>MASNEGVENRPFPYLTVDADLLSNLRQSAAEGLFHSFDLLVGKDAREAGIKFEVLLGVYTNAIQYVRFLETALAVSCVNTEFKDLSRMTDGKIQFRISVPTIAHGDGRRPSKQRTFIVVKNCHKHHISTEMELSMLDLEILHSIPETPVEYAEYVGAVKTVASALQFGVDALERGLINTVLSVKLRHAPPMFILQTLADPTFTERGFSKTVKSDLIAMFKRHLLEHSFFLDRAENMGSGFSQYVRSRLSEMVAAVSGESVLKGVSTYTTAKGGEPVGGVFIVTDNVLRQLLTFLGEEADNQIMGPSSYASFVVRGENLVTAVSYGRVMRTFEHFMARIVDSPEKAGSTKSDLPAVAAGVEDQPRVPISAAVIKLGNHAVAVESLQKMYNDTQSPYPLNRRMQYSYYFPVGLFMPNPKYTTSAAIKMLDNPTQQLPVEAWIVNKNNLLLAFNLQNALKVLCHPRLHTPAHTLNSLNAAPAPRDRRETYSLQHRRPNHMNVLVIVDEFYDNKYAAPVTDIALKCGLPTEDFLHPSNYDLLRLELHPLYDIYIGRDAGERARHRAVHRLMVGNLPTPLAPAAFQEARGQQFETATSLAHVVDQAVIETVQDTAYDTAYPAFFYVVEAMIHGFEEKFVMNVPLVSLCINTYWERSGRLAFVNSFSMIKFICRHLGNNAISKEAYSMYRKIYGELIALEQALMRLAGSDVVGDESVGQYVCALLDPNLLPPVAYTDIFTHLLTVSDRAPQIIIGNEVYADTLAAPQFIERVGNMDEMAAQFVALYGYRVNGDHDHDFRLHLGPYVDEGHADVLEKIFYYVFLPTCTNAHMCGLGVDFQHVAQTLAYNGPAFSHHFTRDEDILDNLENGTLRDLLEISDLRPTVGMIRDLSASFMTCPTFTRAVRVSVDNDVTQQLAPNPADKRTEQTVLVNGLVAFAFSERTRAVTQCLFHAIPFHMFYGDPRVAATMHQDVATFVMRNPQQRAVEAFNRPEQLFAEYREWHRSPMGKYAAECLPSLVSISGMTAMHIKMSPMAYIAQAKLKIHPGVAMTVVRTDEILSENILFSSRASTSMFIGTPNVSRREARVDAVTFEVHHEMASIDTGLSYSSTMTPARVAAITTDMGIHTQDFFSVFPAEAFGNQQVNDYIKAKVGAQRNGTLLRDPRTYLAGMTNVNGAPGLCHGQQATCEIIVTPVTADVAYFQKSNSPRGRAACVVSCENYNQEVAEGLIYDHSRPDAAYEYRSTVNPWASQLGSLGDIMYNSSYRQTAVPGLYSPCRAFFNKEELLRNNRGLYNMVNEYSQRLGGHPATSNTEVQFVVIAGTDVFLEQPCSFLQEAFPALSASSRALIDEFMSVKQTHAPIHYGHYIIEEVAPVRRILKFGNKVVF[4x];>[4x]MARRLPKPTLQGRLEADFPDSPLLPKFQELNQNNLPNDVFREAQRSYLVFLTSQFCYEEYVQRTFGVPRRQRAIDKRQRASVAGAGAHAHLGGSSATPVQQAQAAASAGTGALASSAPSTAVAQSATPSVSSSISSLRAATSGATAAASAAAAVDTGSGGGGQPHDTAPRGARKKQ;>MKVQGSVDRRRLQRRIAGLLPPPARRLNISRGSEFTRDVRGLVEEHAQASSLSAAAVWRAGLLAPGEVAVAGGGSGGGSFSWSGWRPPVFGDFLIHASSFNNAEATGTPLFQFKQSDPFSGVDAVFTPLSLFILMNHGRGVAARVEAGGGLTRMANLLYDSPATLADLVPDFGRLVADRRFHNFITPVGPLVENIKSTYLNKITTVVHGPVVSKAIPRSTVKVTVPQEAFVDLDAWLSGGAGGGGGVCFVGGLGLQPCPADARLYVALTYEEAGPRFTFFQSSRGHCQIMNILRIYYSPSIMHRYAVVQPLHIEELTFGAVACLGTFSATDGWRRSAFNYRGSSLPVVEIDSFYSNVSDWEVIL[2x];>[4x]MDLKVVVSLSSRLYTDEIAKMQQRIGCILPLASTHGTQNVQGLGLGQVYSLETVPDYVSMYNYLSDCTLAVLDEVSVDSLILTKIVPGQTYAIKNKYQPFFQWHGTGSLSVMPPVFGREHATVKLESNDVDIVFPMVLPTPIAEEVLQKILLFNVYSRVVMQAPGNADMLDVHMHLGSVSYLGHHYELALPEVPGPLGLALLDNLSLYFCIMVTLLPRASMRLVRGLIRHEHHDLLNLFQEMVPDEIARIDLDDLSVADDLSRMRVMMTYLQSLASLFNLGPRLATAAYSQETLTATCWLR;> MDVHIDNQVLSGLGTPLLVHLFVPDTVMAELCPNRVPNCEGAWCQTLFSDRTGLTRVCRVFAARGMLPGRPSHRGTFTSVPVYCDEGLPELYNPFHVAALRFYDEGGLVGELQIYYLSLFEGAKRALTDGHLIREASGVQESAAAMQPIPIDPGPPGGAGIEHMPVAAAQVEHPKTYDLKQILLEITQEENRGEQRLGHAGSPALCLGLRLRAGAETKAAAETSVSKHHPALENPSNIRGSAGGEGGGGRAGTGGTVGVGSGALSRVPVSFSKTRRAIRESRALVRGIAHIFSPHALYVVTYPELSAQGRLHRMTAVTHASPATDLAEVSILGAPEREFRFLISVALRISASFREKLAMQAWTAQQEIPVVIPTSYSRIYKNSDLIREAFFTVQTRVSWESCWVKATISNAPKTPDACLWIDSHPLYEEGASAWGKVIDSRPPGGLVGAASQLVALGTDGHCVHLATTSDGQAFLVLPGGFVIKGQLALTPEERGYILARHGIRREQ;>[2x]MALSGHVLIDPARLPRDTGPELMWAPSLRNSLRVSPEALELAEREAERARSERWDRCAQVLKNRLLRVELDGIMRDHLARAEEIRQDLDAVVAFSDGLESMQVRSPSTGGRSAPAPPSPSPAQPFTRLTGNAQYAVSISPTDPPLMVAGSLAQTLLGNLYGNINQWVPSFGPWYRTMSANAMQRRVFPKQLRGNLNFTNSVSLKLMTEVVAVLEGTTQDFFSDVRHLPDLQAALILSVAYLLLQGGSSHQQRPLPASREELLELGPESLEKIIADLKAKSPGGNFMILTSGNKEARQSIAPLNRQAAYPPGTFADNKIYNLFVGAGLLPTTAALNVPGAAGRDRDLVYRIANQIFGEDVPPFSSHQWNLRVGLAALEALMLVYTLCETANLAEAATRRLHLSSLLPQAMQRRKPAMASAGMPGAYPVQTLFRHGELFRFIWAHYVRPTVAADPQASISSLFPGLVLLALELKLMDGQAPSHYAINLTGQKFDTLFEIINQKLLFHDPAAMLAARTQLRLAFEDGVGVALGRPSPMLAAREILERQFSASDDYDRLYFLTLGYLASPVAPS;>MSNGDWGQSQRTRGTGPVRGIRTMDVNAPGGGSGGSALRILGTASCNQAHCKFGRFAGIQCVSNCVLYLVKSFLAGRPLTSRPELDEVLDEGARLDALMRQSGILKGHEMAQLTDVPSSVVLRGGGRVHIYRSAEIFGLVLFPAQIANSAVVQSLAEVLHGSYNGVAQFILYICDIYAGAIIIETDGSFYLFDPHCQKDAAPGTPAHVRVSTYAHDILQYVGAPGAQYTCVHLYFLPEAFETEDPRIFMLEHYGVYDFYEANGSGFDLVGPELVSSDGEAAGTPGADSSPPVMLPFERRIIPYNLRPLPSRSFTSDSFPAARYSPAKTNSPPSSPASAAPASAAPASAAPASAAPASAAPASAAPASAAPASAAPASSPPLFIPIPGLGHTPGVPAPSTPPRASSGAAPQTPKRKKGLGKDSPHKKPTSGRRLPLSSTTDTEDDQLPRTHVPPHRPPSAARLPPPVIPIPHQSPPASPTPHPAPVSTIAPSVTPSPRLPLQIPIPLPQAAPSNPKIPLTTPSPSPTAAAAPTTTTLSPPPTQQQPPQSAAPAPSPLLPQQQPTPSAAPAPSPLLPQQQPPPSAARAPSPLPPQQQPLPSATPAPPPAQQLPPSATTLEPEKNHPPAADRAGTEISPSPPFGQQPSFGDDASGGSGLVRYLSDLEEPFLSMSDSEEAESDLASDIPTTEDEDMFEDEVFSNSLESGSSAPTSPITLDTARSQYYQTTFDIETPEMDFVPLESNIARIAGHTYQEQAIVYDPASNREVPEADALSMIDYLLVTVVLEQGLIRSRDRSSVLNLLEFLKDWSGHLQVPTLDLEQLLTSELNIQNLANMLSENKGRAGEFHKHLAAKLEACLPSLATKDAVRVDAGAKMLAEIPQLAESDDGKFDLEAARRRLTDLLSGGDQEAGEGGGEPEDNSIYRGPHVDVPLVLDDESWKRLLSLAEAARTAVARQQAGVDEEDVRFLALLTAIEYGAPPAASVPPFVHNVAVRSKNAALHVRRCTADIRDKVASAASDYLSYLEDPSLPTVMDFDDLLTHLRHTCQIIASLPLLNIRYTSIEWDYRELLYLGTALSDMSGIPWPLERVEEDDPSIAPLPEFETVAKKQKELETTRENEKRLRTILDDIEAMLGLAGVASAPGAPISPASPSATPANHDNPEATPPLADTAALTIPVIEKYIANAGSIVGAAKNPTYIRLRDTIQQIVRSKKYLMNILKSITFYTIDNYIASFEESIDHLYRDLPVLDPEVQDGIDRILDPMVSEALHTFEMGNRLTLEPARLVALQNFATHSTLKETAAAVNLLPGLLAVYDATITGQAPEDALRLLSGLQNQLSQTLIPGKLKKRFLSYLQKLKNNNNDQLRQKEVQAWRLEAEGFKPATEEQLEAFLDTAPNKELKRQYEKKLRQLMETGRKEKEKLREQEDKERQERRAREANEAWARIRKALGARPEPAPTSPDDWNTLLASLLPDNTDSAAAAAAAVARNTDILDSLTQILAAMLLGITRVRRERLRSLLVDDGGAAERMEAAEPGWFTDIETGPLARLDAWPATPAATAKEGGGGRGAEEAAGALFRARTAADAIRSALAQTRQALQSPDMKSAVVNTDLEAPYAEYERGLAGLLEKRRAAEAALTAIVSEYVDRTLPEATNDPGQANLPPPPTIPQATAPPRLASDSALWPKKPQLLTRRERDDLLQATGDFFSELLTEAEAAEVRALEEQVRESQTLMAKAHEMAASTRRGFHTALEAVLSRSRDEAPDDELRSLLPSPPKAPVQAPLEAALARAAAGNGSWPYRKSLAAAKWIRGICEAVRGLSEGALALAGGAGAWLNLAAAADGEIHELTRLLEVEGMAQNSMDGMEELRLALATLDPKRVAGGKETVADWKRRLSRLEAIIQEAQEESQLQGTLQDLVTQARGHTDPRQLKIVVEAAR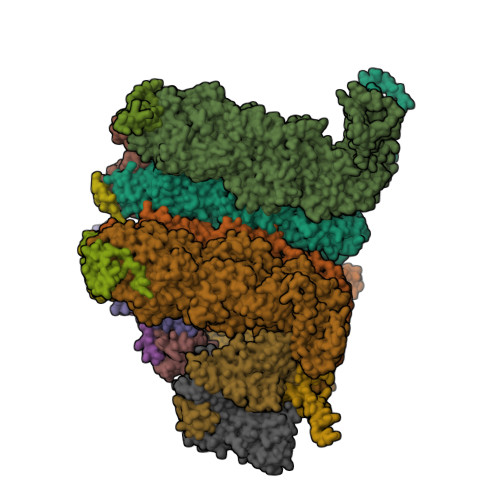GLALGASAGSQYALLKDKLLRYASAKQSFLAFYETAQPTVFVKHPLTNNLPLLITISAPPTGWGNGAPTRRAQFLAAAGPAKYAGTLWLETESPCDPLNPAYVSADTQEPLNYIPVYHNFLEYVMPTVLENPEAFSLTPAGRPQAIGPPQDDQERRRRTLASVASARLSAAAADSYWDTWPDVESNAGELLREYVSAPKALMEDLADNPIVAMTLLAHASLIASRNHPPYPAPATDREVILLEQREMMALLVGTHPAYAAAFLGAPSFYAGLGLVSALARDGGLGDLLSDSVLTYRLVRSPASGRGGMPSTTRGSNDGEDARRLTRHRIAGPPTGFIFFQDAWEEMDTRAALWPHPEFLGLVHNQSTARARACMLLLARRCFAPEALQQLWHSLRPLEGPVAFQDYLRDFVKQAYTRGEELPRAEGLEVPRETPSSYGTVTGRALRNLMPYGTPITGPKRGSGDTIPVSVFEAAVAAAFLGRPLTLFVSSQYLFNLKTLGQVRVVAPLLYCDGHSEPFRSLVETISLNFLQDLDGYSESFEPEMSIFARQAVWLRELLTEARAAKPKEARPPTVAILANRKNIIWKCFTYRHNLPDVQFYFNAAGASRWPTDVLNPSFYEHEDPPLPVGYQLPPNPRNVQELFSGFPPRVGHGLVSGDGFQSADNTPASSDRLQQLGGGETDQGEKGSTTAESEASGPPSPQSPLLEKVAPGRPRDWLSPTSSPRDVTVTPGLAAPITLPGPRLMARPYFGAETRASESPDRSPGSSPRPWPKDSLELLPQPAPQQPPSSPWASEQGPIVYTLSPHSTPSTASGSQKKHTIQIPGLVPSQKPSYPPSAPYKPGQSTGGIAPTPSAASLTTFGLQPQDTQASSQDPPYGHSIMQREKKQQGGREEAAEIRPSATRLPTAVGLRPRAPVVAAGAAASATPAFDPGEAPSGFPIPQAPALGSGLAAPAHTPVGALAPRPQKTQAQRPQDAAALPTPTIKAVGARPVPKATGALAAGARPRGQPTAAPPSAASPPRVSLPVRSRQQQSPAIPLPPMHSGSEPGARPEVRLSQYRHAGPQTYTVRKEAPPSAASQLPKMPKCKDSMYYPPSGSARYPAPFQALSFSQSVASPAPSSDQTTLLWNTPSVVTQFLSIEDIIREVVTGGSTSGDLVVPSGSPSSLSTAAPEQDLRYSLTLSQASRVLSRFVSQLRRKLERSTHRLIADLERLKFLYL[2x]> ANVVEGKFHVTGGN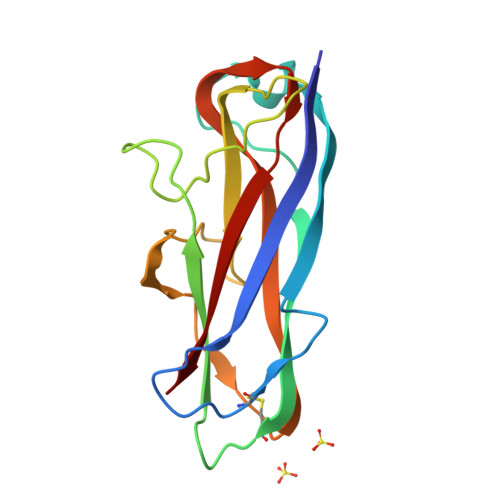VTTAAAACAVDAGSVDQTVQLGQVRTASLAQEGATSSAVGFNIQLNDCDTNVASKAAVAFLGTAIDAGHTNVLALQSSAAGSATNVGVQILDRTGAALTLDGATFSSETTLNNGTNTIPFQARYFATGAATPGAANADATFKVQYQ{3-[(1R)-1-[({(2S)-1-[(2S)-2-cyclohexyl-2-(3,4,5-trimethoxyphenyl)acetyl]piperidin-2-yl}carbonyl)amino]-3-(3,4-dimethoxyphenyl)propyl]phenoxy}acetic acid | C42 H54 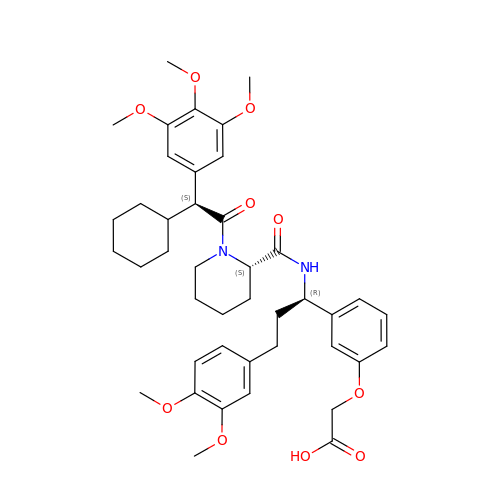N2 O10 | HVSNNDISDMAIJE-XEAFTEEUSA-N> MASWSHPQFEKGSTSAFNPRDTVTVYFHAIVSRHFGFNPEEHKVYVRGGEGLGQKGWTDACEMYCTQDLHDLGSLVEGKMDIPRQSLDKPIPYKYVIHRGGSSKDTVEYEFIYEQAQKKGEHVNRCLRVVSTSLGNGDWHQYDDIICMRSTGFFQQAKNRILDSTRKELLKGKKQAAVVMLDRIFSVLQPWSDINLQSFMTQFLQFYSVVREPMIHDGRARKWTSLQYEEKEVWTNLWEHVKKQMAPFLEGKSGESLPADCPVRSKLTLGLSILFMVEAAEFTVPKKDLDSLCYLLIPSAGSPEALHSDLSPVLRIRQRWRIYLTNLCLRCIDERCDRWLGILPLLHTCMQKSPPKKNSKSQPEDTWAGLEGISFSEFRDKAPTRSQPLQFMQSKMALLRVDEYLFRSWLSVVPLESLSSYLENSIDYLSDVPVRVLDCLQGISYRLPGLRKISNQNMKKDVENVFKMLMHLVDIYQHRIFGENLLQIYLTECLTLHETVCNITANHQFFEIPALSAELICKLLELSPPGHTDEGLPEKSYEDLVTSTLQEALATTRNWLRSLFKSRMLSISSAYVRLTYSEEMAVWRRLVEIGFPEKHGWKGSLLGDMEGRLKQEPPRLQISFFCSSQCRDGGLHDSVSRSFEKCVIEAVSSACQSQTSVLEGLSCQDLQKFGTLLSAVITKSWPVHNGEPVFDVDEIFKYLLKWPDVRQLFELCGTNEKIIDNITEEGRQLMATAESVFQKVAGELENGTIVVGQLELILEHQSQFLDIWNLNRRRLPSQEKACDVRSLLKRRRDDLLFLKQEKRYVESLLRQLGRVKHLVQVDFGNIEIIHSQDLSNKKLNEAVIKLPNSSSYKRETHYCLSPDIREMASKLDSLKDSHIFQDFWQETAESLNTLDKDPRELKVSLPEVLEYLYNPCYDNFYTLYENLKSGKITFAEVDAIFKDFVDKYDELKNDLKFMCTMNPQDQKGWISERVGQIKEYHTLHQAVSSAKVILQVRRALGVTGDFSVLNPLLNFADSFEDFGNEKLDQISPQFIKAKQLLQDISEPRQRCLEELARQTELVAWLHKALEDINELKVFVDLASISAGENDIDVDRVACFHDAVQGYASLLYKMDERTNFSDFMNHLQELWRALDNDQHLPDKLKDSARNLEWLKTVKESHGSVELSSLSLATAINSRGVYVIEAPKDGQKISPDTVLRLLLPDGHGYPEALRTYSTEELKELLNKLMLMSGKKDHNSNTEVEKFSEVFSNMQRLVHVFIKLHCAGNMLFRTWTAKVYCCPDGGIFMNFGLELLSQLTEKGDVIQLLGALCRQMEDFLDNWKTVVAQKRAEHFYLNFYTAEQLVYL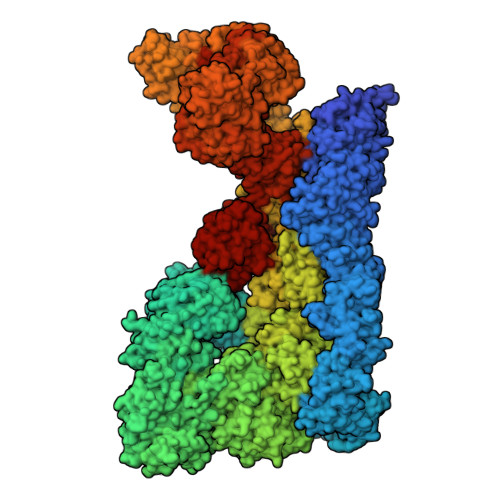SSELRKPRPSEAALMMLSFIKGKCTVQDLVQATSACESKADRYCLREVMKKLPQQLLSEPSLMGKLQVIMMQSLVYMSAFLPHCLDLDALGRCLAHLATMGGTPVERPLPKGLQAGQPNLILCGHSEVLPAALAIYMQAPRQPLPTFDEVLLCTPATTIEEVELLLRRCLTSGSQGHKVYSLLFADQLSYEVGCQAEEFFQSLCTRAHREDYQLVILCDAAREHCYIPSTFSQYKVPLVPQAPLPNIQAYLQSHYQVPKRLLSAATVFRDGLCVGIVTSERAGVGKSLYVNTLHTKLKAKLRDETVPLKIIRLTEPHLDENQVLSALLPFLKEKYQKMPVIFHIDISTSVQTGIPIFLFKLLILQYLMDINGKIWRRSPGHLYLVEIPQGLSVQPKRSSKLNARAPLFKFLDLFPKVTCRPPKEVIDMELTPERSHTDPAMDPVEFCSEAFQRPYQYLKRFHQQQNLDTFQYEKGSVEGSPEECLQHFLIYCGLINPSWSELRNFAWFLNCQLKDCEASIFCKSAFTGDTLRGFKNFVVTFMILMARDFATPTLHTSDQSPGRQSVTIGEVVEEDLAPFSLRKRWESEPHPYVFFNGDHMTMTFIGFHLETNNNGYVDAINPSNGKVIKKDVMTKELFDGLRLQRVPFNIDFDNLPRYEKLERLCLALGIEWPIDPDETYELTTDNMLKILAIEMRFRCGIPVIIMGETGCGKTRLIKFLSDLKRGSVEAETMKLVKVHGGTTPSMIYSKVKEAERTAFSNKAQHKLDTILFFDEANTTEAVSCIKEILCDRTVDGEHLHEDSGLHIIAACNPYRKHSQEMILRLESAGLGYRVSAEETADRLGSIPLRQLVYRVHALPPSLIPLVWDFGQLNDSAEKLYIQQIVQRLVDSVSVNPSETCVIADVLSASQMFMRKRENECGFVSLRDVERCVKVFRWFHDHSDMLLKELDKFLHESSDSTHTFERDPVLWSLVMAIGVCYHASLEEKASYRTAIARCFPKPYNSSRAILDEVTHVQDLFLRGAPIRTNIARNLALKENVFMMVICIELKIPLFLVGKPGSSKSLAKIIVADAMQGQAAFSELFRCLKQVHLVSFQCSPHSTPQGIISTFKQCARFQQGKDLGQYVSVVVLDEVGLAEDSPKMPLKTLHPLLEDGCIEDDPAPYKKVGFVGISNWALDPAKMNRGIFVSRGSPNEKELIESAEGICSSDRLVQDKIRGYFAPFAKAYETVCQKQDKEFFGLRDYYSLIKMVFAKAKASKRGLSPQDITHAVLRNFSGKDNIQALSIFTASLPEARYKEEVSTVELIKQNIYPGPQASSRGLDGAESRYLLVLTRNYVALQILQQTFFEGQQPEIIFGSSFPQDQEYTQICRNINRVKICMETGKMVVLLNLQNLYESLYDALNQYYVYLGGQKYVDLGLGTHRVKCRVHTAFRLIVIEEKDVVYKQFPVPLINRLEKHYLDMNTVLQPWQKSIVQELQQWAHEFADVKADQFIARHKYSPADVFIGYHSDACASVVLQAVERQGCRDLTEELYRKVSEEARSILLDCATPDAVVRLSGSSLGSFTAKQLSQEYYYAQQHNSFVDFLQAHLRMTHHECRAVFTEITTFSRLLTGNDCDVLASELRGLASKPVVLSLQQYDTEYSFLKDVRSWLTNPGKRKVLVIQADFDDGTRSAQLVASAKYTAINEINKTQGTKDFVFVYFVTKLSRMGSGTSYVGFHGGLWRSVHIDDLRRSTIMASDVTKLQNVTISQLFKPEDKPEQEEMEIETSQSKELAEEQMEVEDSEEMKKASDPRSCDCSQFLDTTRLVQSCVQGAVGMLRDQNESCARNMRRVTILLDLLNEDNTRNASFLRESKMRLHVLLNKQEENQVRSLKEWVTREAANQDALQEAGTFRHTLWKRVQDVVTPILASMIAHIDRDGNLELLAQPDSPAWVQDLWMFIYSDIKFLNISLVLNNTRSNSEMSFILVQSHMNLLKDAYNAVPFSWRIRDYLEELWVQAQYITDTEGLSKKFVEIFQKTPLGVFLAQFPVAQQQKLLQSYLKDFLLLTMKVSSREELMFLQMALWSCLRELQEASGTPDETYKFPLSLPWVHLAFQHFRTRLQNFSRILTIHPQVLSSLSQAAEKHSLAGCEMTLDAFAAMACAEMLKGDLLKPSPKAWLQLVKNLSTPLELVCSEGYLCDSGSMTRSVIQEVRALWNRIFSIALFVEHVLLGTESHIPELSPLVTTYVSLLDKCLEEDSNLKTCRPFVAVMTTLCDCKDKASKKFSRFGIQPCFICHGDAQDPVCLPCDHVYCLRCIQTWLIPGQMMCPYCLTDLPDKFSPTVSQDHRKAIEKHAQFRHMCNSFFVDLVSTMCFKDNTPPEKSVIDTLLSLLFVQKELLRDASQKHREHTKSLSPFDDVVDQTPVIRSVLLKLLLKYSFHEVKDYIQNYLTQLEKKAFLTEDKTELYLLFISCLEDSVHQKTSAGCRNLEQVLREEGHFLRTYSPGLQGQEPVRIASVEYLQEVARVRLCLDLAADFLSELQEGSELAEDKRRFLKHVEEFCTRVNNDWHRVYLVRKLSSQRGMEFVQSFSKQGHPCQWVFPRKVIAQQKDHVSLMDRYLVHGNEYKAVRDATAKAVLECKTLDIGNALMACRSPKPQQTAYLLLALYTEVAALYRSPNGSLHPEAKQLEAVNKFIKESKILSDPNIRCFARSLVDNTLPLLKIRSANSILKGTVTEMAVHVATILLCGHNQILKPLRNLAFYPVNMANAFLPTMPEDLLVHARTWRGLENVTWYTCPRGHPCSVGECGRPMQESTCLDCGLPVGGLNHTPHEGFSAIRNNEDRTQTGHVLGSPQSSGVAEVSDRGQSPVVFILTRLLTHLAMLVGATHNPQALTVIIKPWVQDPQGFLQQHIQRDLEQLTKMLGRSADETIHVVHLILSSLLRVQSHGVLNFNAELSTKGCRNNWEKHFETLLLRELKHLDKNLPAINALISQDERISSNPVTKIIYGDPATFLPHLPQKSIIHCSKIWSCRRKITVEYLQHIVEQKNGKETVPVLWHFLQKEAELRLVKFLPEILALQRDLVKQFQNVSRVEYSSIRGFIHSHSSDGLRKLLHDRITIFLSTWNALRRSLETNGEIKLPKDYCCSDLDLDAEFEVILPRRQGLGLCGTALVSYLISLHNNMVYTVQKFSNEDNSYSVDISEVADLHVISYEVERDLNPLILSNCQYQVQQGGETSQEFDLEKIQRQISSRFLQGKPRLTLKGIPTLVYRRDWNYEHLFMDIKNKMAQSSLPNLAISTISGQLQSYSDACEALSIIEITLGFLSTAGGDPGMDLNVYIEEVLRMCDQTAQVLKAFSRCQLRHIIALWQFLSAHKSEQRLRLNKELFREIDVQYKEELSTQHQRLLGTFLNEAGLDAFLLELHEMIVLKLKGPRAANSFNPNWSLKDTLVSYMETKDSDILSEVESQFPEEILMSSCISVWKIAATRKWDRQSRGGGHHHHHHHHHH>[5x]EDRLFKHLFRGYNR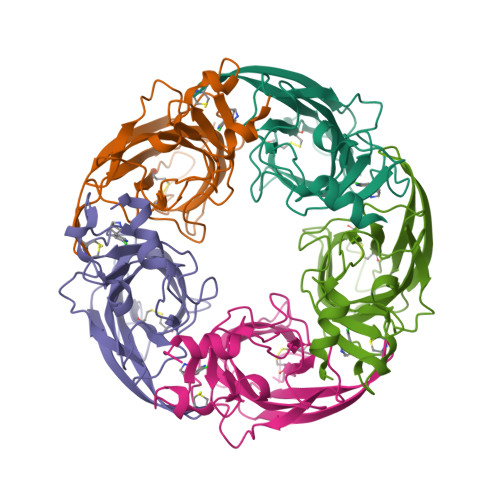WARPVPNTSDVVIVRFGLSIAQLIDVDEKNQMMTTNVWLKQEWSDYKLRWNPTDFGNITSLRVPSEMIWIPDIVLYNNADGEFAVTHMTKAHLFSTGTVHWVPPAIYKSSCSIDVTFFPFDQQNCKMKFGSWTYDKAKIDLEQMEQTVDLKDYWESGEWAIVNATGTYNSKKYDCCAEIYPDVTYAFVIRRLPHHHHHH>MAAVENFEGYVEPELFERPGTSLPNKLGVMPQLTWPNVLNGTNCEKPAVPNYKPPSKVDVIIIGAGPVGLTTAACLLRQGITVRILDRSPHPLPVGRADGLQPRSMEVFDLLGLGEEVYHVGIRVEHTTVYKDGKQHIFAESHQAPGNEAHYTGLHACTQTEVEHLLIRDLIRHDILVERPCTATSYTFDEEADASVTHPITVNITNEATGAEEVVTARFLVGSDGAHSMIRKSLPIEFPGVKTDLHWGIVDAVINSDFPHRWTFGTVLNSEYGGCLIIPRERNMVRLYVQLRAEPGKAFDHSKWGPEEILVILNKVFAPYTLSYAEPVDWYTILTINERVATSFTYKDRIFLAGDSCHVHSAKGAFGMNTGVMDAHNLAWKLAMLCRGIAKPSLLASYDVERRENALRAVATSARYLRFVGNCTFQAIDGSGEVDKEADELVVPPGEDKDVFYFKKFVGQVGRFLIGLDVDYAENALNKLSPAVSRARAGYRASNPRVALSRSHSGRLYHSFGHLGQFTLLVFASNMGGALNAKLHALDSYLAGPSSFYHAYGGADTFKIVVVVRATPSQADQRVKTFPFLSKAGHTVYDDQLPLSHFGGDAHALYGVSHEEGAIVVVRPDSWIGTSSTISDARSLESYFDGFLFKSTEGSY[4x]

In this work, using activity-guided fractionation together with proteomic analyses, we identify an NADPH/FAD-dependent monooxygenase VibO as the key enzyme performing a crucial ring-expansive oxygenation on the phenol ring to generate the oxepin-2-one structure of 3. The crystal structure of VibO reveals that it forms a dimeric phenol hydroxylase-like architecture featured with a unique substrate-binding pocket adjacent to the bound FAD. Phylogenetic analysis revealed that VibO belongs to group A flavin-dependent monooxygenases and is clustered with type O Baeyer-Villiger monooxygenases and aromatic ring hydroxylases. VibO, on the other hand, acts as an NADPH/FAD-dependent monooxygenase catalyzing oxygenation on the phenol ring of 6 to form the oxepinone 3 in the biosynthetic pathway to vibralactone.

In the crystal structure, each asymmetric unit contains four VibO molecules, which form two symmetric dimers, in line with our analytical ultracentrifugation-based assay. In the dimeric VibO structure, each VibO monomer contains 25 β-strands (β1-β25) and 13 α-helices (α1-α13), and is composed of three distinct sub-domains: the FAD-binding domain (residues 1–127, 141–245 and 336–419), the middle domain (residues 128–140, 246–335 and 420–472), and the C-terminal domain (residues 473–653). The C-terminal domain of VibO adopts a peroxiredoxin-like α/β-fold, which directly packs against the FAD-binding domain and is far away from the middle domain. In particular, the dimerization of VibO is mediated by three different types of sub-domain/sub-domain interactions between the two monomeric VibO molecules (the middle domain/middle domain interaction, the FAD-binding domain/FAD-binding domain interaction and the FAD-binding domain/C-terminal domain interaction), covering a total of ~3436 Å2 surface area. Across the middle and FAD-binding domains of VibO, the co-factor FAD is buried in a solvent-exposed and highly positive-charged pocket. Specifically, the ADP and ribityl groups of the bound FAD are embedded within the FAD-binding domain, whereas its isoalloxazine ring is located at the interface between the middle domain and the FAD-binding domain. Notably, the co-factor FAD in the crystal structure of the VibO/FAD complex adopts an “out”-conformation, suggesting that the bound FAD is located outside of the active site of VibO. Further careful analyses of the VibO structure uncovered that hydrogen bonds and electrostatic interactions are primarily responsible for the specific binding of VibO with FAD, involving the main chains of G66, V68, S89, D356, A363 and M369 as well as the side chains of R88, R97, Q160, R287 and D356 of VibO. Careful structural analyses showed that there is a highly hydrophobic cavity adjacent to the isoalloxazine ring of the bound FAD in the VibO/FAD complex, and importantly, this pocket corresponds to the substrate-binding site of the phenol hydroxylase PHHY.8,8'-[CARBONYLBIS[IMINO-3,1-PHENYLENECARBONYLIMINO(4-METHYL-3,1-PHENYLENE)CARBONYLIMINO]]BIS-1,3,5-NAPHTHALENETRISULFONIC ACID | C51 H40 N6 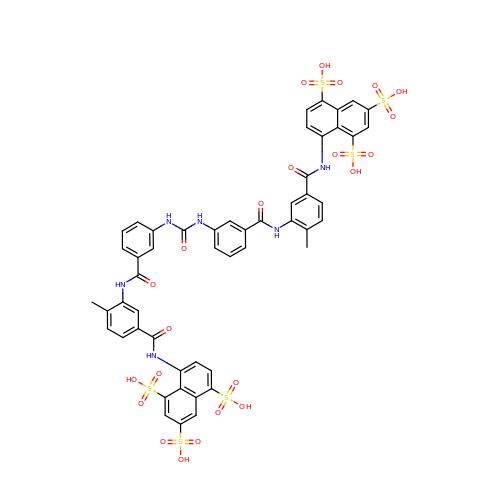O23 S6 | FIAFUQMPZJWCLV-UHFFFAOYSA-N>AQVQQLTPAQQAALRNQQAMAANLQARQIVLQQSYPVIQQVETQTFDPANRSVFDVTPANVGIVKGFLVKVTAAITNNHATEAVALTDFGPANLVQRVIYYDPDNQRHTETSGWHLHFVNTAKQGAPFLSSMVTDSPIKYGDVMNVIDAPATIAAGATGELTMYYWVPLAYSETDLTGAVLANVPQSKQRLKLEFANNNTAFAAVGANPLEAIYQGAGAADCEFEEISYTVYQSYLDQLPVGQNGYILPLIDLSTLYNLENSAQAGLTPNVDFVVQYANLYRYLSTI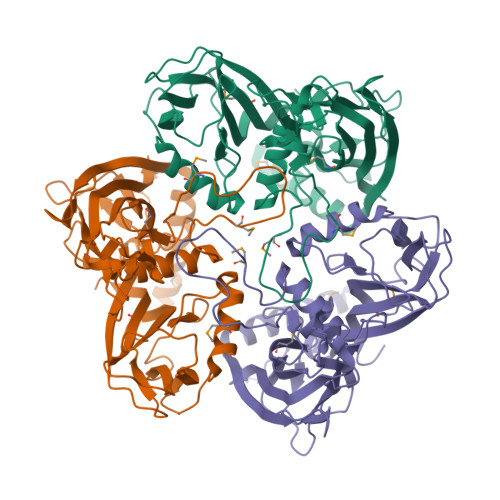AVFDNGGSFNAGTDINYLSQRTANFSDTRKLDPKTWAAQTRRRIATDFPKGVYYCDNRDKPIYTLQYGNVGFVVNPKTVNQNARLLMGYEYFTSRTELVNAGTISTT[3x]>MGDRGPEFVATTVELPLQQKADAAQTVTGPLPFGNSLLKEFVLDPAYRNLNHGSFGTIPSAIQQKLRSYQTAAEARPCPFLRYQTPVLLDESRAAVANLLKVPVETVVFVANATMGVNTVLRNIVWSADGKDEILYFDTIFGACGKTIDYVIEDKRGIVSSRCIPLIYPAEDDDVVAAFRDAIKKSREEGKRPRLAVIDVVSSMPGVRFPFEDIVKICKEEEIISCVDGAQGIGMVDLKITETDPDFLISNCHKWLFTPRGCAVFYVPVRNQHLIRSTLPTSHGFVPQVGNRFNPLVPAGNKSAFVSNFEFVGTVDNSPFFCVKDAIKWREEVLGGEERIMEYMTKLAREGGQKVAEILGTRVLENSTGTLIRCAMVNIALPFVVGEDPKAPVKLTEKEEKDVEGLYEIPHEEANMAFKWMYNVLQDEFNTFVPMTFHRRRFWARLSAQVYLEMSDFEWAGKTLKELCERVAKGEYK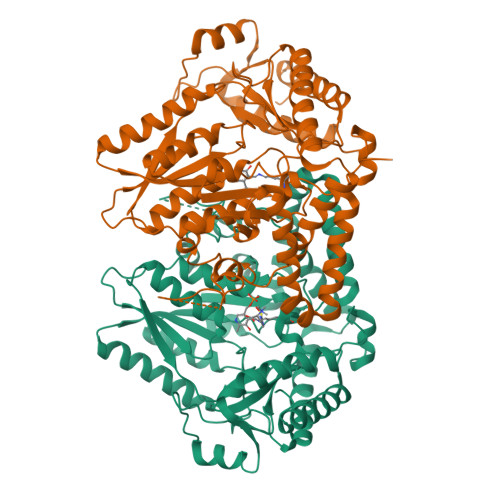ESALEVDLQGDHGLSAWSHPQFEK[8x]> MRNGLVWLLHPALPSTLHSILGARPPPVKRLCGFPKQIYSTMNNPAIQRIEDHIVKSPEDKREYRGLELANGIKVLLISDPTTDKSSAALDVHIGSLSDPPNIPGLSHFCFHMLFLGTKKYPKENEYSQFLSEHAGSSNAFTSGEHTNYYFDVSHEHLEGALDRFAQFFLCPLFDASCKDREVNAVDSEHEKNVMNDAWRLFQLEKATGNPKHPFSKFGTGNKYTLETRPNQEGIDVREELLKFHSTYYSSNLMAICVLGRESLDDLTNLVVKLFSEVENKNVPLPEFPEHPFQEEHLKQLYKIVPIKDIRNLYVTFPIPDLQQYYKSNPGHYLGHLIGHEGPGSLLSELKSKGWVNTLVGGQKEGARGFMFFIINVDLTEEGLLHVEDIILHMFQYIQKLRAEGPQEWVFQECKDLNAVAFRFKDKERPRGYTSKIAGKLHYYPLNGVLTAEYLLEEFRPDLIDMVLDKLRPENVRVAIVSKSFEGKTDRTEQWYGTQYKQEAIPEDVIQKWQNADLNGKFKLPTKNEFIPTNFEILALEKDATPYPALIKDTAMSKLWFKQDDKFFLPKACLNFEFFSPFAYVDPLHCNMAYLYLELLKDSLNEYAYAAELAGLSYDLQNTIYGMYLSVKGYNDKQPILLKKITEKMATFEIDKKRFEIIKEAYMRSLNNFRAEQPHQHAMYYLRLLMTEVAWTKDELKEALDDVTLPRLKAFIPQLLSRLHIEALLHGNITKQAALGVMQMVEDTLIEHAHTKPLLPSQLVRYREVQLPDRGWFVYQRRNEVHNNCGIEIYYQTDMQSTSENMFLELFCQIISEPCFNTLRTKEQLGYIVFSGPRRANGIQGLRFIIQSEKPPHYLESRVEAFLITMEKAIEDMTEEAFQKHIQALAIRRLDKPKKLSAECAKYWGE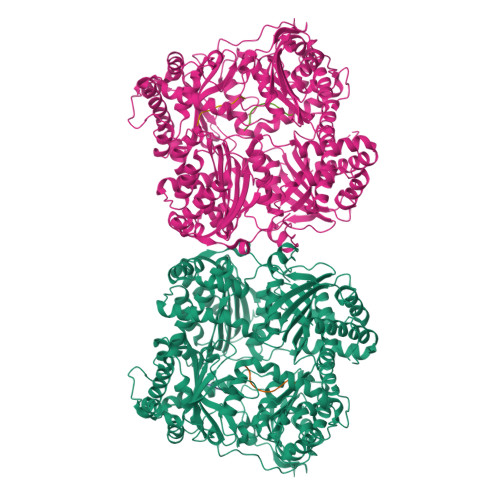IISQQYNYDRDNIEVAYLKTLSKDDIIKFYKEMLAVDAPRRHKVSVHVLAREMDSCPVVGEFPSQNDINLSEAPPLPQPEVIHNMTEFKRGLPLFPLVKPHINFMAAKL> MGNDISLIALLAFSTLLPFIIASGTCFVKFSIVFVMVRNALGLQQIPSNMTLNGVALLLSMFVMWPIMHDAYVYFEDEDVTFNDISSLSKHVDEGLDGYRDYLIKYSDRELVQFFENAQLKRQYGEETETVKRDKDEIEKPSIFALLPAYALSEIKSAFKIGFYLYLPFVVVDLVVSSVLLALGMMMMSPVTISTPIKLVLFV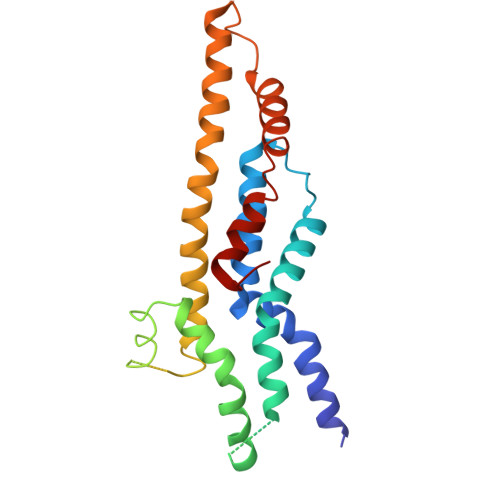ALDGWTLLSKGLILQYMDIAT>GSFVEMVDNLRGKSGQGYYVEMTVGSPPQTLNILVDTGSSNFAVGAAPHPFLHRYYQRQLSSTYRDLRKGVYVPYTQGKWEGELGTDLVSIPHGPNVTVRANIAAITESDKFFINGSNWEGILGLAYAEIARPDDSLEPFFDSLVKQTHVPNLFSLQLCGAGFPLNQSEVLASVGGSMIIGGIDHSLYTGSLWYTPIRREWYYEVIIVRVEINGQDLKMDCKEYNYDKSIVDSGTTNLRLPKKVFEAAVKSIKAASSTEKFPDGFWLGEQLVCWQAGTTPWNIFPVISLYLMGEVTNQSFRITILPQQYLRPVEDVATSQDDCYKFAISQSSTGTVMGAVIMEGFYVVFDRARKRIGFAVSACHVHDEFR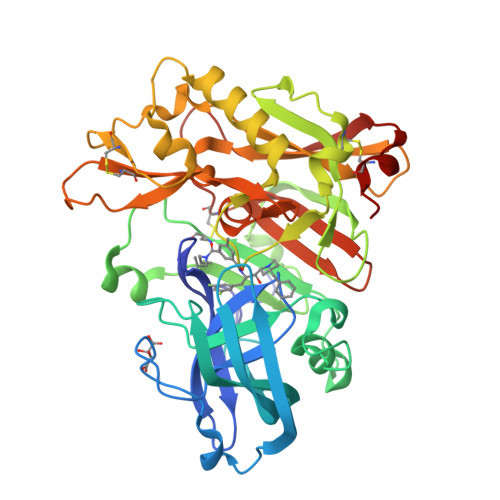TAAVEGPFVTLDMEDCGYNI[2x]N-ethyl-2-[(6-methoxypyridin-3-yl)-(2-methylphenyl)sulfonyl-amino]-N-(pyridin-3-ylmethyl)ethanamide 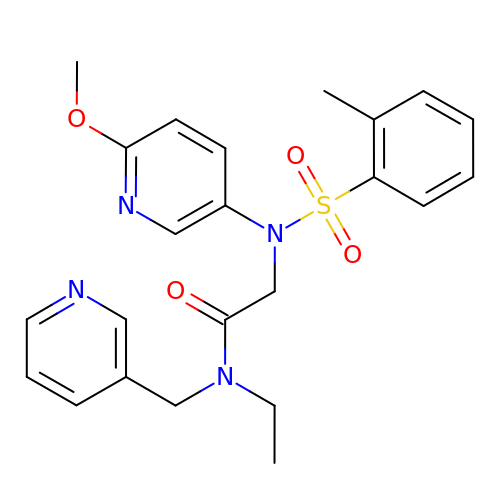| C23 H26 N4 O4 S | KJPHTXTWFHVJIG-UHFFFAOYSA-N>GPHMSELREDIQTKGKEVENFEKNLEECITRITNTEKCLKELMELKTKARELREECRSLRSRCDQLEERVSAAEDEINEIKREGKFREKRIKRNEQSLQEIWDY[6x]

The L1ORF1 protein (L1ORF1p) is known as an RNA-binding protein, whereas the L1ORF2 protein (L1ORF2p) harbors the necessary catalytic functions, consisting of an endonuclease and a reverse transcriptase. Mammalian L1ORF1p has a unique architecture, even among the ORF1ps encoded by non-LTR retrotransposons. It consists of three structural domains, connected by short linkers. These domains are first, a coiled coil domain, which causes the protein to form homotrimers, second, an RRM (RNA recognition motif) domain, and third, a C-terminal domain (CTD), which cooperates with the RRM domain in binding single stranded nucleic acid substrates.

We therefore tried to obtain a detailed crystal structure and indeed, a bacterially expressed fragment of human L1ORF1p, encompassing the entire coiled coil domain (hL1ORF1p-cc) crystallized with two trimers (T1 and T2) present per asymmetric unit, yielding two slightly differing structures of the trimeric human L1ORF1p coiled coil domain at 2.65 Å resolution. Trimer T1 forms an extended rod with an overall length of 150 Å. For the polypeptide chains A and B, all 14 heptads are found in the electron density in a continuously helical, extended conformation. In heptad XII, chain C begins to deviate and breaks the threefold symmetry, and then becomes untraceable in the electron density in heptad XIII. Trimer T2 is highly similar to trimer T1 for heptads II to XI (r.m.s.d. for Cα atoms = 0.781 Å), but, in comparison to trimer T1, heptad XII also remains roughly threefold symmetric. Apparently therefore, the N-terminal heptads of the coiled coil domain are deformable and can switch between an α-helical and an unwound state. Most strikingly, in heptad IX, there is a sharply localized distortion in the helical geometry of both the coiled coil bundle and of the individual polypeptide chains. The distortion is caused by the stammer, which can be precisely assigned to residues M91, E92 and L93. These three residues form an extra 310-helical turn between positions d and e of heptad IX and create an additional hydrophobic core layer (d*) at L93. Arginines (heptad III, R135) are much more rarely observed at d-layers, and especially the combination with a glycine (G132) in the preceding a-layer, where the guanidino groups of R135 coordinate a second chloride ion, is unique so far to the human L1ORF1p.5-[2,3-DICHLORO-4-(5-{1-[2-(2-GUANIDINO-4-METHYL-PENTANOYLAMINO)-ACETYL]-PIPERIDIN-4-YL}-1-METHYL-1H-PYRAZOL-3-YL)-PHENOXYMETHYL]-FURAN-2-CARBOXYLIC 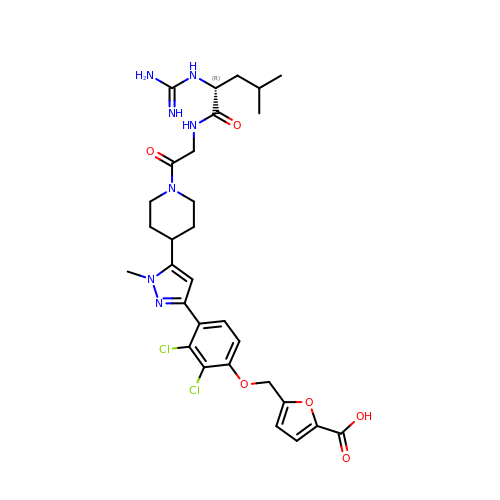ACID | C30 H37 Cl2 N7 O6 | VNZHOIDQBPFEJU-OAQYLSRUSA-N> MKSSHHHHHHENLYFQSNAMSYPGKDKNIPGRIIEALEDLPLSYLVPKDGLAALVNAPMRVSLPFDKTIFTSADDGRDVNINVLGTANSTTSSIKNEAEKERLVFKRPSNFTSSANSVDYVPTNFLEGLSPLAQSVLSTHKGLNDSINIEKKSEIVSRPEAKHKLESVTSNAGNLSFN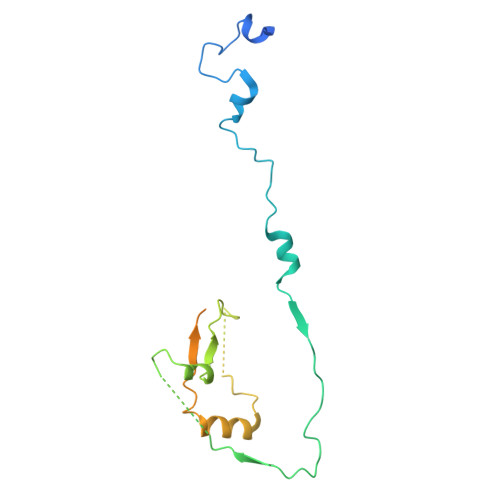DNSSNKKTKTSTGVTMTQANLA> GVTKNNSCKKVGVEELINEKGCDLMIIRINRCRGHCFSFTFPNPLTKKYSVHAKCCRMVEW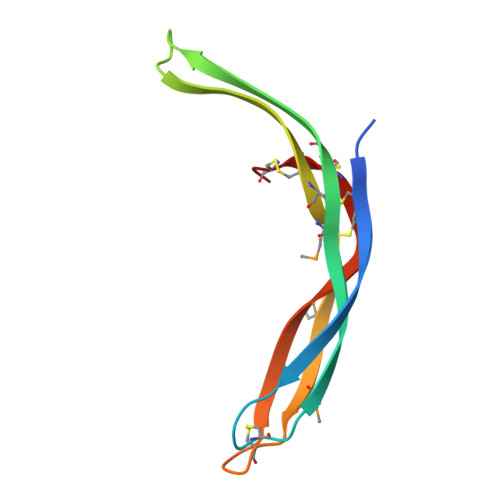EMLETELKCSKGNRNLRIPSATQCECFDCLV(2S)-({N-[(3S)-3-({N-[(2S,4E)-2-ISOPROPYL-7-METHYLOCT-4-ENOYL]-L-LEUCYL}AMINO)-2-OXOHEXANOYL]GLYCYL}AMINO)(PHENYL)ACETIC 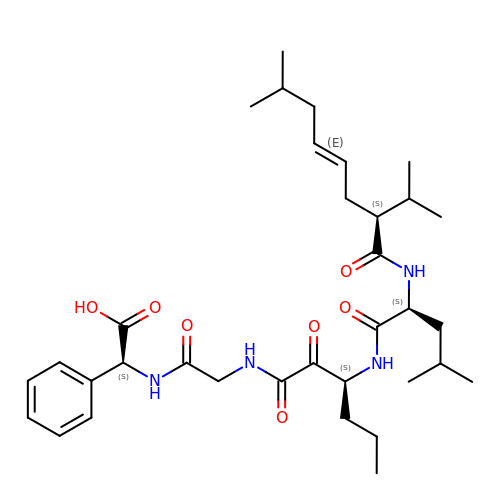ACID | C34 H52 N4 O7 | KWTWSYDWITXSOY-IMAVGDMBSA-N> PLQPIPGVASVSPANGAVVGVAHPVVVTFTTPVTDRRAVERSIRISTPHNTTGHFEWVASNVVRWVPHRYWPPHTRVSVGVQELTEGFETGDALIGVASISAHTFTVSRNGEVLRTMPASLGKPSRPTPIGSFHAMSKERTVVMDSRTIGIPLNSSDGYLLTAHYAVRVTWSGVYVHSAPWSVNSQGYA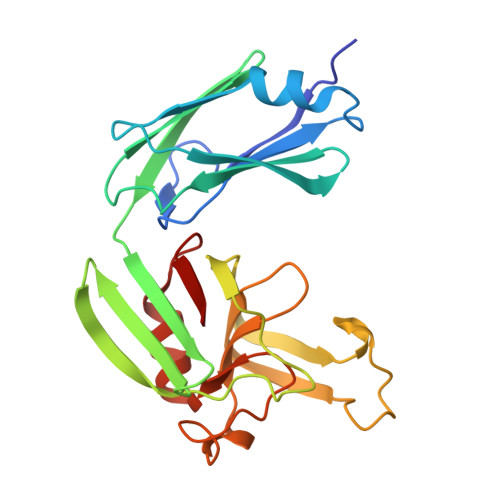NVSHGCINLSPDNAAWYFDAVTVGDPIEVVG> MLQKRIPQIICTLLLLGSFSQIKAQDRVPFDQGKKYTLAKVSVVGKISFNEQTVVTFSGLQKGQEITVPGEEITSAIKKLGKLGLFDEIAFYINKVENDSIYLDLNIVELPKLNEVKITGVKKSKVEGLIKDNNLTKNKIVNENLITTTKNYIENKYKKDGFYNTKVVITTTPDTTAGNQVNMLVRVDKGDKVKISSIDFTGNKQLSDSKLRAAMKDTKQKNVLRVFKASKFIPEKYKTDLEKVIASYKEKGYRDARIIYDSVIYNKKKNMLAIKIDVEEGNKYYFGNIKFLGNTVYSDQQLNRYLGIKKGETYNGVLLEKRIADNTKPDGEDITNLYQNNGYLFSKINAVEVKTVNDTIDFEIRITEGPIAYFNKIYVTGNDKTNDHVIYRELRTKPGNKYSKEELVRTIREIGQLGFFDPESIKPEFRNVDPAAGTVDIEYQLVEKGSSQVELQGGYGGGGFIGTLGLSFNNFSARKLFDKDAYKPLPMGDGQKVALRLQGSTYFQTYSLSFSEPWFGGKKPVQFSSSISYSKQFNYNYSSRDVNRNQSFNIFTVQVGLAKRLTVPDDYFVLSQSVSYQHYDLNNYYTGLFTFGNGASRNLAYTIGLSRSNKGVNPIFPTYGSEFSISAKVTPPYSLFNNI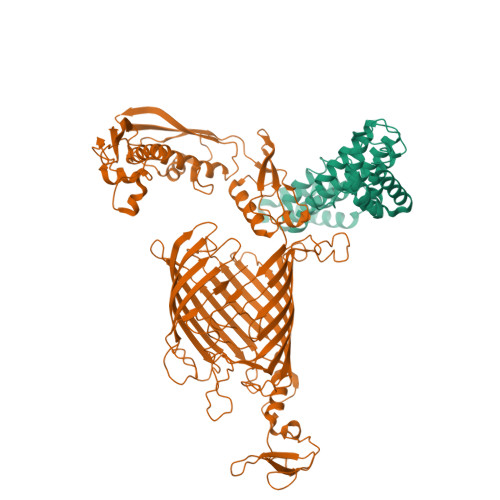NYGDLQNQKEYKTQYTGTTTTTGIDGQAINPGDYTKTETVNGQSGTVSVGSDYKSADTDVGKVDQKKYNWLEYYKVKFKADWYTKIYGKLVLRTLTEFGFLGAYDQSRGVVPFERFYLGGDGMANYSMDGRETIQLRGYPNNSLTPIIEDRNSSRYGQQIGATIYNKFSMELRYPITLKSSASIYALTFLEAGSSYPTFKDYNPFDLNRSAGAGLRVFMPAFGLLGIDFGYGFDALPGSTTNKANGWETHFIIGQQF;> MKKIVSLLIVAALFCSCSEYQKALKNEDVAAKFEVATKMYDAGKYNKAIRLFEQLAPTYRGKPQAEKLFYMFSQSYYKTKQYYLAGYQFESFVSGYPRSEKVQEAAFLGAYSYSKLAPVYSLDQADTVKALDKLQAFIDNYPNSEYLAQANESVKILNGKLEKKAYENAKGYNTISDYKSALVAFDNFIADFPGTPLKEDALFYKYDSAYQLAINSVPSKMEERLHVAQTAYANLMKYKSDTKYKEKADQMNARVETDLQKFTK2-[2-(2-ethylphenoxy)ethanoyl-[[4-(1,2,4-triazol-1-yl)phenyl]methyl]amino]-~{N}-methyl-ethanamide | C22 H25 N5 O3 | 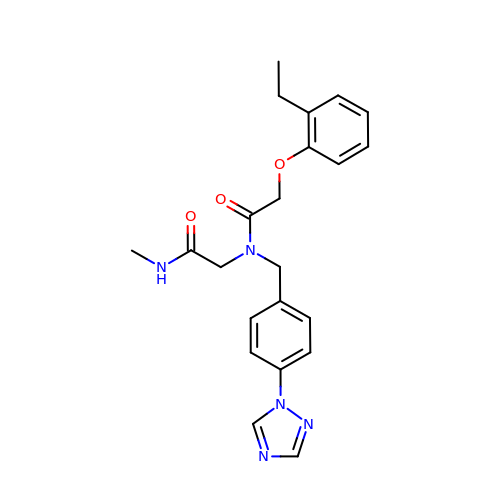DUJWKHCSHDYNGS-UHFFFAOYSA-N>MQWSGARALEALLTVAGELRGPPLQLDTGQLLKIAKRGGVTAVEAVHAWRNALTGAPLNLTPEQVVAIASHDGGKQALETVQRLLPVLCQAHGLTPQQVVAIASHDGGKQALETVQRLLPVLCQAHGLTPEQVVAIASHDGGKQALETVQALLPVLCQAHGLTPEQVVAIASNGGGKQALETVQRLLPVLCQAHGLTPQQVVAIASNGGGKQALETVQRLLPVLCQAHGLTPQQVVAIASRGGGKQALETVQRLLPVLCQAHGLTPQQVVAIASNNGGKQALETVQRLLPVLCQAHGLTPQQVVAIASHDGGKQALETVQRLLPVLCQAHGLTP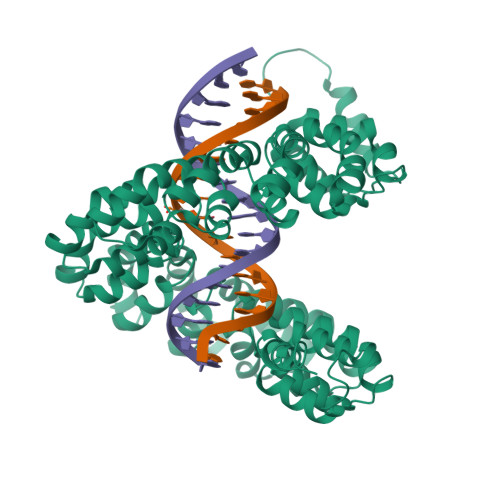QQVVAIASNNGGKQALETVQRLLPVLCQAHGLTPEQVVAIASNGGGKQALETVQRLLPVLCQAHGLTPEQVVAIASHDGGKQALETVQRLLPVLCQAHGLTPQQVVAIASNGGGRPALESIVAQLSRPDPALAALTNDHLVALACLGGRPALDAVKKLEHHHHHH[4x]> MSFLISFDKSKKHPAHLQLANNLKIALALEYASKNLKPEVDNDNAAMELRNTKEPFLLFDANAILRYVMDDFEGQTSDKYQFALA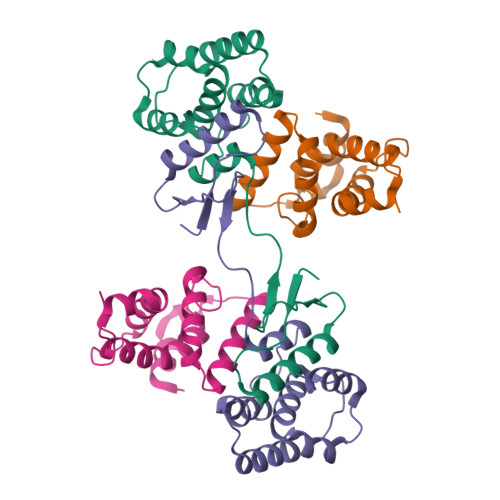SLQNLLYHKELPQQHVEVLTNKAIENYLVELKEPLTTTDLILFANVYALNSSLVHSKFPELPSKVHNAVALAKKH;> MSDLVTKFESLIISKYPVSFTKEQSAQAAQWESVLKSGQIQPHLDQLNLVLRDNTFIVSTLYPTSTDVHVFEVALPLIKDLVASSKDVKSTYTTYRHILRWIDYMQNLLEVSSTDKLEINHD>[2x]GPGSSDETIFDLPPYIKVFKDGRVERLHSSPYVPPSLNDPETGGVSWKDVPISSVVSARIYLPKINNHDEKLPIIVYFHGAGFCLESAFKSFFHTYVKHFVAEAKAIAVSVEFRLAP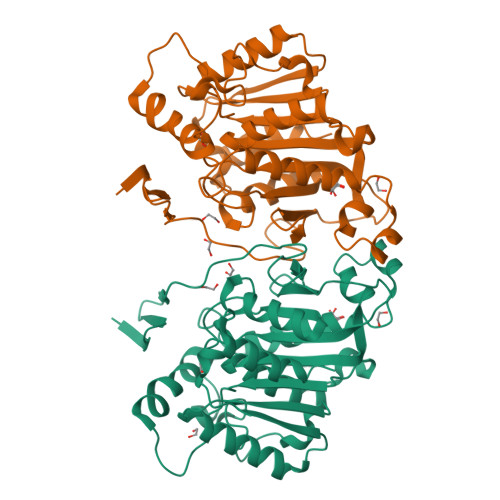ENHLPAAYEDCWEALQWVASHVGLDISSLKTCIDKDPWIINYADFDRLYLWGDSTGANIVHNTLIRSGKEKLNGGKVKILGAILYYPYFLIRTSSKQSDYMENEYRSYWKLAYPDAPGGNDNPMINPTAENAPDLAGYGCSRLLISMVADEARDITLLYIDALEKSGWKGELDVADFDKQYFELFEMETEVAKNMLRRLASFIK N-(4-fluorobenzoyl)-L-alloisoleucyl-O-[(S)-{[(1S)-1,3-dicarboxypropyl]amino}(hydroxy)phosphoryl]-L-serine | C21 H29 F 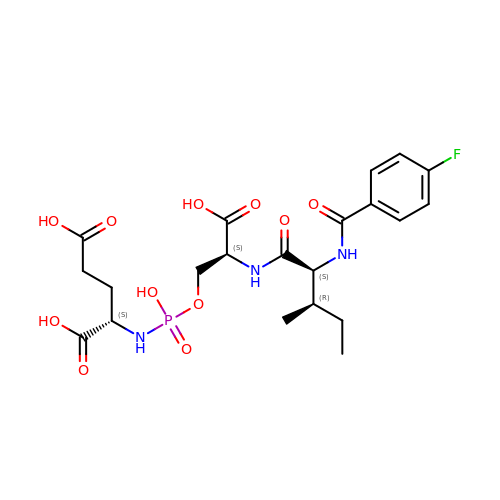N3 O11 P | RRPCLWZKRJZYQY-ZUFFMMDNSA-N> ISEFMAKIETLEEALKAAEALEREGVHAILDLLGEMVRTEEEARAFQRGLLELVWALAGKPWPKYISLKLTQLGLDLSEDLALALLREVLREAEPRGVFVRLDMEDSPRVEATLRLYRALREEGFSQVGIVLQSYLYRTEKDLLDLLPYRPNLRLVKGAYREPKEVAFPDKRLIDAEYLHLGKLALKEGLYVAFATHDPRIIAELKRYTEAMGIPRSRFEFQFLYGVRPEEQRRLAREGYTVRAYVPYGRDWYPYLTRRIAERPENLLLVLRSLVSGLE

Proline dehydrogenase (ProDH, EC 1.5.5.2) is a ubiquitous flavoenzyme involved in proline catabolism. It oxidises L-proline to Δ1-pyrroline-5-carboxylate (P5C), which is non-enzymatically hydrolysed to glutamic semialdehyde (GSA). ProDH adopts a distorted (βα)8 TIM-barrel fold. Next to methylenetetrahydrofolate reductase (MTHFR), ProDH is the only known TIM-barrel enzyme that contains an FAD cofactor.

We created a TtProDH variant (ΔABC), which lacks the N-terminal helices αA, αB and αC. ΔABC is poorly active but binds the flavin cofactor in stoichiometric amounts. From this variant, the MBP-tag could be successfully removed and the purified ProDH fragment was used for crystallisation. The three-dimensional model for TtProDH ΔABC comprises residues 38–279. Using ESI-MS, we detected that the C-terminal helix α8 of MBP-TtProDH ΔABC is unstable and becomes proteolytically cleaved in E. coli after Thr287. Deletion of the last 22 residues might increase the flexibility of the remaining C-terminal end of the protein and explain why residues 280–287 are not visible in the crystal structure. For the FAD cofactor, no electron density was observed for the adenosine 5′-monophosphate (AMP) moiety. This suggests that either the AMP part of the FAD shows multiple orientations and therefore is highly mobile, or that (part of) the bound cofactor is FMN instead of FAD. The mode of binding of the FMN-part of the flavin cofactor is strictly conserved compared to that of TtProDH. To confirm that ΔABC binds both FMN and FAD, the flavin content of TtProDH ΔABC was determined using fluorescence and mass spectroscopy for holo-EE. This revealed that TtProDH ΔABC contains 78 ± 5% FMN and 22 ± 5% FAD, similar as for holo-EE. The TtProDH variant ΔABC reveals that helices αA, αB, αC and α8 are not essential for binding of the flavin cofactor in TtProDH.>MWRYPRNADQTFWAFRTCQRQSEGAKSLREWYRWNLPNDEDTHCYVKCVWLHLGLYNEQNKSLRVDRIMEQFNSRSVAIPGGINTISGPTDGTCKDIYDKTINFFNNNVNDLRTAFYGIKKLSDEWFTQNSNTKPKGTKISDFCNAENREKGGADCQHACSAYYYRLVDEDNEP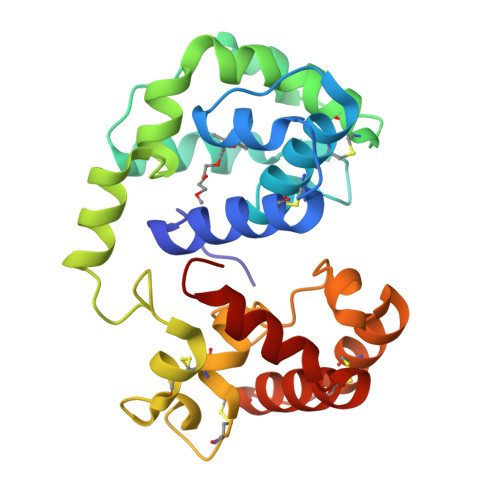IHFRNLNILGITDEQFASCVKASKNKQGCKVADTMYNCVEKHNSQALKILDNQSPTY[2x]>SGSGSSDEEFKFLATEAKMLITAAERLAGTDPELQEMVALIKKELEQAERTFRNGDKSEAQRQLEFVLTAARAVMNVAAAANAAGTDPELIEMVLRILKQLKEAIRTFQNGDQEEAETQLRFVLRAAIAVAVVAAALVLAGTDPELQEMVKQILEELKQAIETFARGDKEKALTQLLFVAWAAHAVAMIAAAANLAGTDPRLQQQVKEILEKLKEAIETFQKGDEEQAFRQLAEVLAEAALVALRAALTN[4x]

To investigate the photophysics of special pairs independently of the complexities of native photosynthetic proteins, and as a first step toward creating synthetic photosystems for new energy conversion technologies, we designed C2-symmetric proteins that hold two chlorophyll molecules in closely juxtaposed arrangements. For Chl dimer protein scaffolds, we chose hyperstable C2-symmetric repeat protein dimers containing symmetric pockets with tunable sizes and geometries. In this dimeric repeat protein architecture, the hydrophobic core is independent of the small molecule-binding site, enabling full customization for binding with little impact on the overall protein structure. We describe de novo-designed proteins that hold Chl dimers in precisely defined, closely juxtaposed geometries.

SP2 was intended to assemble a ZnPPaM dimer with a conformation substantially different from that of native special pairs to investigate the effect of dimer geometry. The SP2 crystal structure was solved in both the apo state and the ZnPPaM-bound state to 2.4 and 2.5 Å resolution, respectively. The apo- and holo-state amino acid backbones both agree with the SP2 design model to within 1.4 Å r.m.s.d. The holo-state crystal structure has two copies of the SP2 dimer in the asymmetric unit; alignment of the two ZnPPaM dimers shows that their binding geometries are equivalent, with an r.m.s.d of 0.22 Å over the tetrapyrrole rings. Despite the accuracy of the protein backbone design, the crystal structure shows that the ZnPPaM molecules are rotated and translated relative to the design model (3.5 Å r.m.s.d. across tetrapyrrole ring atoms). Compared with the apo-state crystal structure, the SP2 binding cavity widens by ~1.6 Å in the presence of ZnPPaM; this expansion provides the extra volume needed for the ZnPPaM molecules to adopt their unexpected conformation. While the ZnPPaM dimer in SP2 differs from the design model, the crystal structure nevertheless satisfies the objective of creating a non-native dimer geometry. Using the SP2−ZnPPaM dimer crystal structure, we calculated an excitonic coupling energy of 241 cm−1. The experimental SP2−ZnPPaM absorption features at 668 and 690 nm correspond to a Qy peak splitting of 477 cm−1 (a coupling of 239 cm−1), which is consistent with the calculated value. The close agreement between the calculated and experimental data supports the conclusion that the SP2−ZnPPaM dimer system exhibits excitonic delocalization.>[8x]MSLTLFHNPASPYVRKVMVLLHETGQLNRVALQASQLSPVAPDAALNQDNPLGKIPALRLDNGQVLYD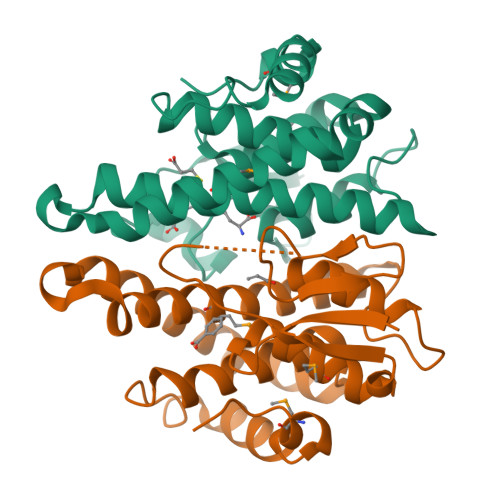SRVILDYLDQQHVGNPLIPRDGSARWRRLTLAALADGIMDASVLVRYELALRAPEKHWEQWLDGQRDKIRRALAVLEAEAIAELASHFDIAAISVACALGYLDFRHPDLEWRQDHPQLAAWYFEISQRPSMLATRPPVEGHHHHHH Titin is a protein expressed in the skeletal and cardiac, or striated, muscle of vertebrates that plays various roles in muscle structure and function. Encoded by the gene TTN, titin spans half a sarcomere (the basic contractile unit of muscle) and has various functions including preventing sarcomere over-extension (Gautel and Djinović-Carugo, 2016), acting as a molecular ruler for thick filament formation and as a hub for numerous signalling molecules (Kruger and Linke, 2011, Linke and Hamdani, 2014). Fn3 domains are only found in the A-band region of titin, where they are arranged with Ig domains in a pattern termed super-repeats, which themselves are repeated. Fn3 domains have a characteristic beta sandwich fold, with a core of hydrophobic residues as the “filling” between two beta sheets that pack against each other face-to-face.

Fn3-3 and Fn3-11 are found in the non-repetitive region of A-band titin near the tip of the thick filament, Fn3-20 is in the second D-zone super-repeat and Fn3-49, Fn3-56, Fn3-85 and Fn3-90 are located in the 1st, 2nd, 6th and 7th C-zone super-repeats, respectively. Fn3-20 is at position 6 of the D-zone super-repeat, and Fn3-49, Fn3-56, Fn3-85 and Fn3-90 are at the 11th, 10th, 6th and 2nd position of the C-zone super-repeat, respectively. Alignment of their primary sequences show an insert in Fn3-20 extending the loop connecting strands C'/D to E by five residues that does not align with residues in any other titin Fn3 domain. The extended loop in Fn3-20 results in a unique protrusion from the back “side” of the domain, not present in the other structures presented here, nor any other titin Fn3 domain structurally determined. All domains determined present a typical Fn3 domain fold, with the extended loop connecting strands C’/D and E in Fn3-20 being the largest difference between the structures. With this extended loop only present in one further domain (Fn3-25), this could be a candidate for a (semi-) unique binding site on a titin Fn3 domain for a putative ligand, analogous to the “KTLE loop” in Ig-159 (A169) required for MuRF1 binding to titin. The structures increase the coverage of titin’s primary sequence with experimentally determined high resolution structural information by ∼ 15% and nearly double the coverage of A-band titin, with the first experimental structure from the D-zone (Fn3-20). The variant in Fn3-20, Leu18237Pro, was identified in a patient also carrying two C-terminal truncating variants inherited in trans, whilst Val22232Glu in Fn3-49 was co-inherited in trans with a truncating variant in the kinase domain at the A-band / M−band junction. Fn3-20 Leu18237Pro was solubly expressed but caused a 16.9 °C reduction in domain thermal stability.

> GSSLPGPPGKPKVLARTKGSMLVSWTPPLDNGGSPITGYWLEKREEGSPYWSRVSRAPITKVGLKGVEFNVPRLLEGVKYQFRAMAINAAGIGPPSEPSDPEVAGDPIF> MNFESIISHMNDHHKSNLVDLCKKFGGIEQVQDVFLKSVDFNGLDLVYNDKENLRVEFPKKADENTIKDTIISLCMSAKSEQNFSGVEKELNEFMLSFNSVALATLNANGEVVCSYAPFVSTQWGNYIYISEVSEHFNNIKVNPNNIEIMFLEDESKAASVILRKRLRYRV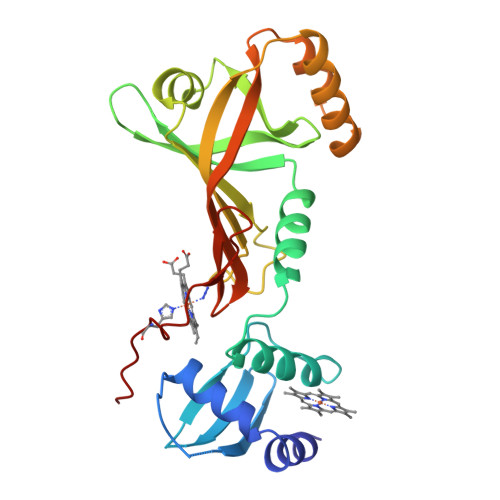NASFLERGERFDQIYDEFEKQTGGEGGIKTIRKMLDFHLVKLEFKKGRFVKGFGQAYDIENGNVTHVGASGNPHKFLHKH>GYDLSDVNTDDAVMGESWVAPLGMGYVTSDDVVNVEKVPSIREVDGAYVMIYDGEMKIKGKSLRAASDKVEIASEDITTGDIDGLFDGDFVLALTNPHITLKSNVKNASLDCSLSIEAENTSKKEATSSDFTLSTVSPNIWIGPLDPKTDAFKFVKNEKLPGIVQIVPQKIHLSLSADSKQWTNAPADALSELRYAVELPLTPAPEFSAVSVERIEDAFDEDFVDYIFSDGSARIYGEVTNEMPFDMSIEMVIMDE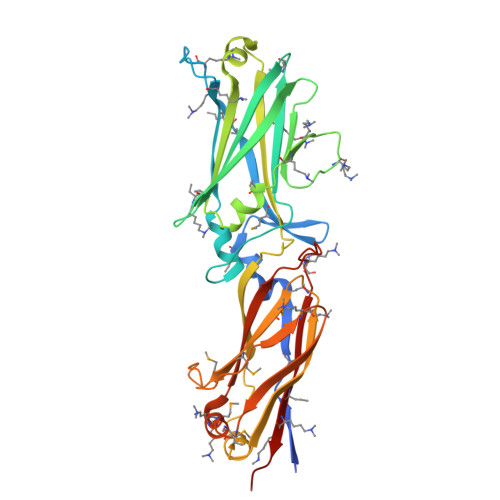NNVPVDIQFPAQEVKGQSGEVIFEITKEDMPKMKDARHIDLNLHLTGRDQGEALKKGQKTTFNLKLKKEGGISI[2x]>MNNTIINSLIGGDDSIKRSNVFAVDSQIP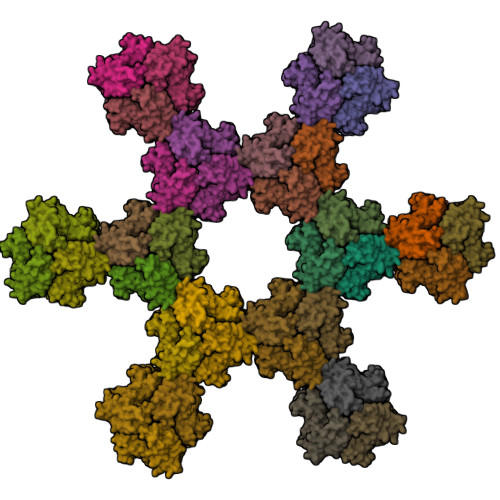TLYMPQYISLSGVMTNDGPDNQAIASFEIRDQYITALNHLVLSLELPEVKGMGRFGYVPYVGYKCINHVSISSCNGVIWEIEGEELYNNCINNTIALKHSGYSSELNDISIGLTPNDTIKEPSTVYVYIKTPFDVEDTFSSLKLSDSKITVTVTFNPVSDIVIRDSSFDFETFNKEFVYVPELSFIGYMVKNVQIKPSFIEKPRRVIGQINQPTATVTEVHAATSLSVYTKPYYGNTDNKFISYPGYSQDEKDYIDAYVSRLLDDLVIVSDGPPTGYPESAEIVEVPEDGIVSIQDADVYVKIDNVPDNMSVYLHTNLLMFGTRKNSFIYNISKKFSAITGTYSDATKRTIFAHISHSINIIDTSIPVSLWTSQRNVYNGDNRSAESKAKDLFINDPFIKGIDFKNKTDIISRLEVRFGNDVLYSENGPISRIYNELLTKSNNGTRTLTFNFTPKIFFRPTTITANVSRGKDKLSVRVVYSTMDVNHPIYYVQKQLVVVCNDLYKVSYDQGVSITKIMGDNN[6x]> MNITKPFPLPTGYFGIPLGLAALSLAWFHLENLFPAARMVSDVLGIVASAVWIL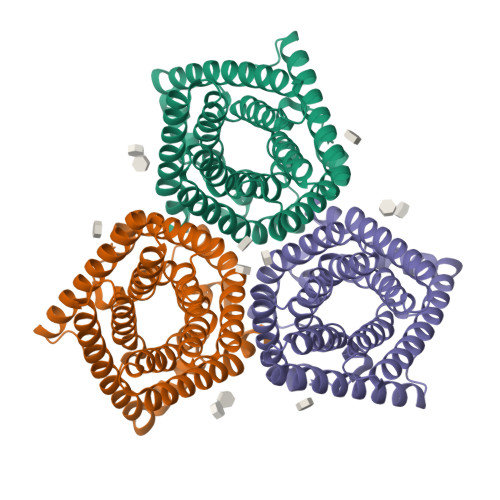FILMYAYKLRYYFEEVRAEYHSPVRFSFIALIPITTMLVGDILYRWNPLIAEVLIWIGTIGQLLFSTLRVSELWQGGVFEQKSTHPSFYLPAVAANFTSASSLALLGYHDLGYLFFGAGMIAWIIFEPVLLQHLRISSLEPQFRATMGIVLAPAFVCVSAYLSINHGEVDTLAKILWGYGFLQLFFLLRLFPWIVEKGLNIGLWAFSVGLASMANSATAFYHGNVLQGVSIFAFVFSNVMIGLLVLMTIYKLTKGQFFLK> SAFAP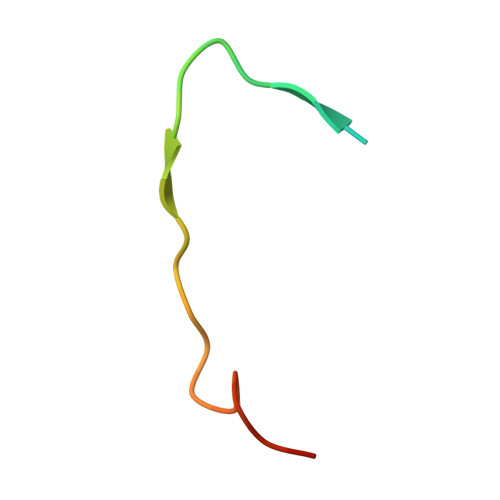DFKELDENVEYEERESEFDIED>[10x]MRALIVYTELTDKDSVISHAVARLASELNDEHVETVIIRDFEDGLAYIRSNTSIDCLLYGRDMSDRDEQIQAHRLITQLHRRQEDVPVFLLSDREEALVAFDRNMMEQVDEFAWILEDSADFIAGRVLAAIQRYRSQLLPPLMKSLIKYSDVHEYSWAAPGHQGGVGFTKTPAGRIYHDFFGENLFRTDIGIERVAVGSLLDHTGAFGECEKNAARIFGADQSYSVVVGTSGSNRTIMQACMTDDDVVVIDRNCHKSIEQGLILTGAKPVYMIPSRNRYGIIGPIYPKEMTPDAIKFKIAANPLTKGKVKQKPAYSVVTNCTYDGVCYNARKVQDLLDGSLDRIHFDEAWYGYARFNPLYRNHFAMRDEERTENEPTIFATHSTHKLLNALSQASFIHVRNGRNAIDFNRFNQAYLMHSTTSPLYAICASNDIAADMMDGNSG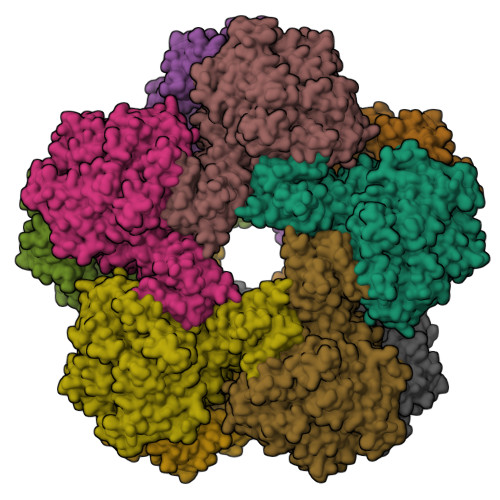RSLTDEVIRESIDFRQSLAYLYKEFLNDDEWFFKPWNQEMVKDPATGKRYAFEDAPVELLMREQSCWVMHPEDKWHGFNDIPDNWAMLDPIKVSILAPGMGDDGKLLDTGVPAALVTAWLNHYGIVPTRTTDFQIMFLFSMGITKGKWGTLVNTLLSFKRHYDNNTALKKVLPEVVASAPEIYGEMGLRDLGDKMFAYLQKNNPGARLNQAYSQLPQVMMTPRDAYQQIVANRVEAVPVDQLMGRVAANSIIPYPPGIPMLLSGENFGDENSPHIHYLRSLQAWDSEFPGFEHETEGTEIIDGQYYVMCVKTCDE>[2x]GSHMASMKKKGSVVIVGRINLSGDTAYAQQTRGEEGCQETSQTGRDKNQVEGEVQI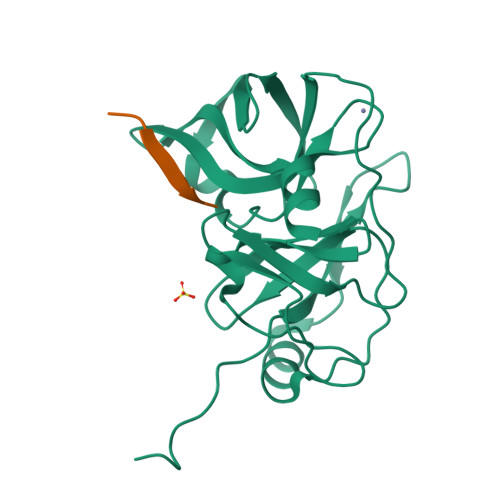VSTATQTFLATSINGVLWTVYHGAGTRTIASPKGPVTQMYTNVDKDLVGWQAPQGSRSLTPCTCGSSDLYLVTRHADVIPVRRRGDSRGSLLSPRPISYLKGSAGGPLLCPAGHAVGIFRAAVSTRGVAKAVDFIPVESLETTMRSP;>XTEDVVCC[2x]>MEMDIRFRGDDDEALARALLKMVVRAVSFGAQVRFTDDGNDLEIRITGVPEQVLKELAK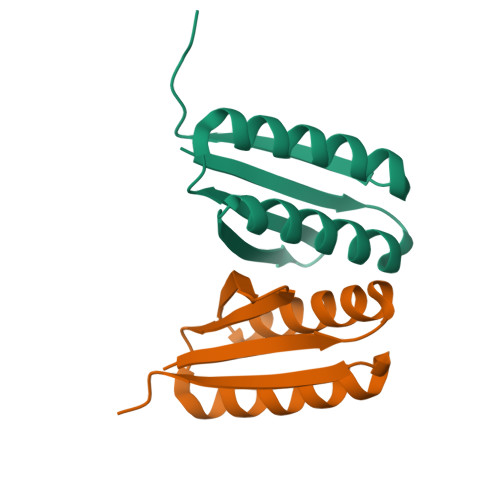EAERLAKEFGITVTRTIRGSLEHHHHHH[4x]> SNALTAEEIIQYISDAKKFTPIKVYLNGNFEGITYPESFKVFGSE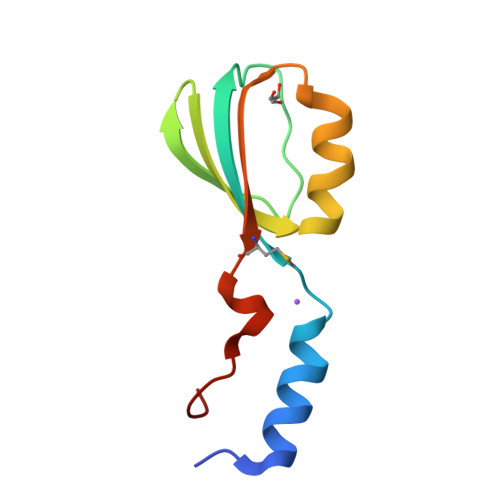QSKVIFCEADDWKPFYEAYGSQFEDIEIEMDRRNSAIPLKDL>GPHMPGSGQIQLWQFLLELLSDSANASCITWEGTNGEFKMTDPDEVARRWGERKSKPNMNYDKLSRALRYYYDKN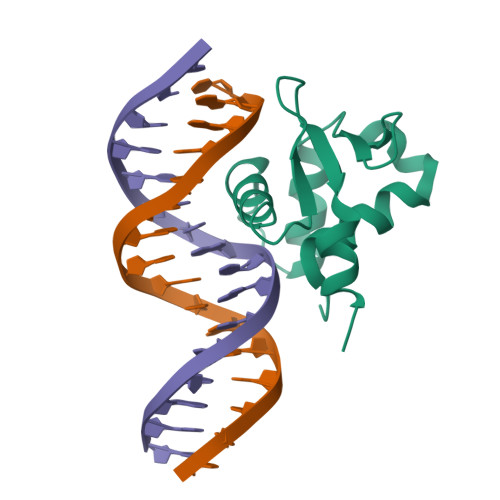IMTKVHGKRYAYKFDFHGIAQALQPHPTE[2x]6-ACETAMIDO-6-DEOXY-CASTANOSPERMINE | C10 H18 N2 O4 | 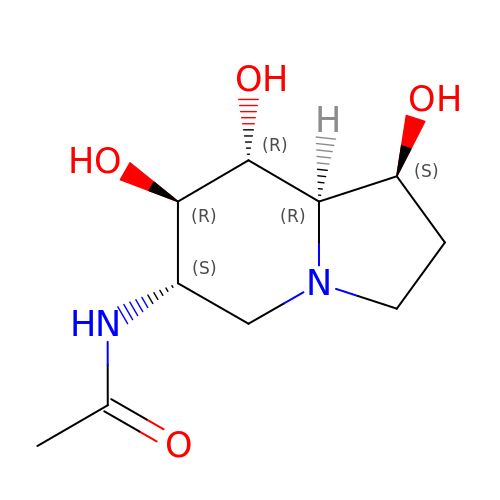IHKWXDCSAKJQKM-SRQGCSHVSA-N> GPLGSEFPFDVDALFPERITVLDQHLRPPARRPGTTTPARVDLQQQIMTIIDELGKASAKAQNLSAPITSASRMQSNRHVVYILKDSSARPAGKGAIIGFIKVGYKKLFVLDDREAHNEV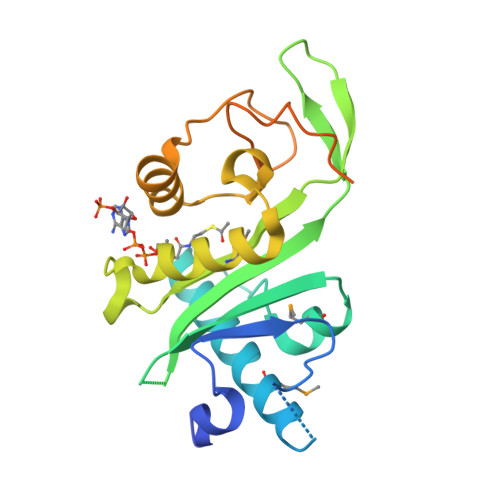EPLCILDFYIHESVQRHGHGRELFQYMLQKERVEPHQLAIDRPSQKLLKFLNKHYNLETTVPQVNNFVIFEGFFAHQHRPPAPSLRATRHSRAAAVDPTPAAPARKLPPKRAEGDIKPYS> MMLPDWKIRKEILIEPFNEKSLQPAGYDLRVGKEAYINGRLINVEKEGKV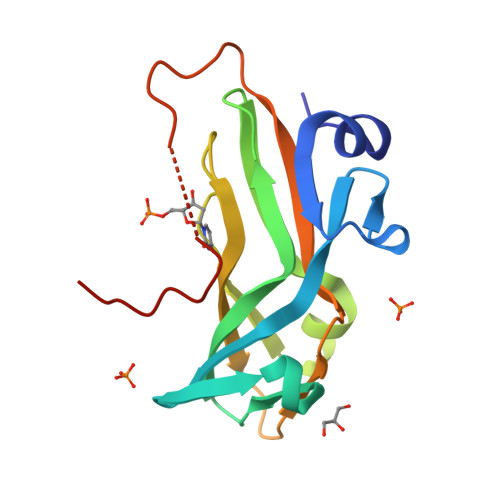VIPPKTHALILTLERVKLPDDVMGDMKLRSSLAREGLLGSFAWVDPGWDGNLTLMLFNASEEPVELNYGERFVQIAFIRLEGPAKNPYRGNYQGSQHLVLSKRRK> MVSSAQMGFNLQALLEQLSQDELSKFKYLITTFSLAHELQKIPHKEVDKADGKQLVEILTTHCDSYWVEMASLQVFEKMHRMDLSERAKDEVREAALKSFNKRKPLSLGITRKERPPLDVDEMLERFKTEAQAFTETKGNVICLGKEVFKGKKPDKDNRCRYILKTKFREMWKSWPGDSKEVQVMAERYKMLIPFSNPRVLPGPFSYTVVLYGPAGLGKTTLAQKLMLDWAEDNLIHKFKYAFYLSCRELSRLGPCSFAELVFRDWPELQDDIPHILAQARKILFVIDGFDELGAAPGALIEDICGDWEKKKPVPVLLGSLLNRVMLPKAALLVTTRPRALRDLRILAEEPIYIRVEGFLEEDRRAYFLRHFGDEDQAMRAFELMRSNAALFQLGSAPAVCWIVCTTLKLQMEKGEDPVPTCLTRTGLFLRFLCSRFPQGAQLRGALRTLSLLAAQGLWAQTSVLHREDLERLGVQESDLRLFLDGDILRQDRVSKGCYSFIHLSFQQFLTALFYTLEKEEEEDRDGHTWDIGDVQKLLSGVERLRNPDLIQAGYYSFGLANEKRAKELEATFGCRMSPDIKQELLRCDISCKGGHSTVTDLQELLGCLYESQEEELVKEVMAQFKEISLHLNAVDVVPSSF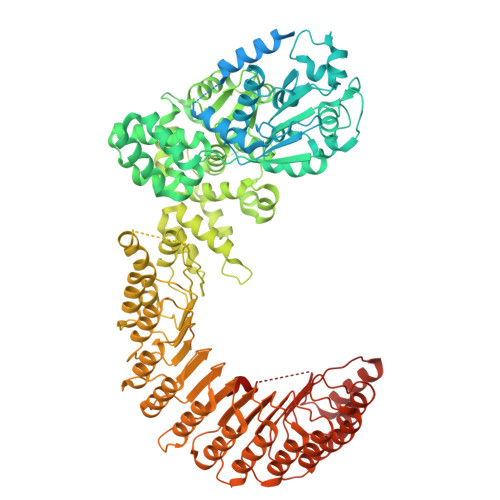CVKHCRNLQKMSLQVIKENLPENVTASESDAEVERSQDDQHMLPFWTDLCSIFGSNKDLMGLAINDSFLSASLVRILCEQIASDTCHLQRVVFKNISPADAHRNLCLALRGHKTVTYLTLQGNDQDDMFPALCEVLRHPECNLRYLGLVSCSATTQQWADLSLALEVNQSLTCVNLSDNELLDEGAKLLYTTLRHPKCFLQRLSLENCHLTEANCKDLAAVLVVSRELTHLCLAKNPIGNTGVKFLCEGLRYPECKLQTLVLWNCDITSDGCCDLTKLLQEKSSLLCLDLGLNHIGVKGMKFLCEALRKPLCNLRCLWLWGCSIPPFSCEDLCSALSCNQSLVTLDLGQNPLGSSGVKMLFETLTCSSGTLRTLRLKIDDFNDELNKLLEEIEEKNPQLIIDTEKHHPWAERPSSHDFMI> MSDQPRPTVIITGASSGVGLYATKALANRGWHVIMACRNLEKAEQAAKNLQIPPEAYTILHLDLSSLASVRGFVESFRALNRPLRALVCNAAVYYPLLKEPIYSVDGYEITVATNHLGHFLLINLLL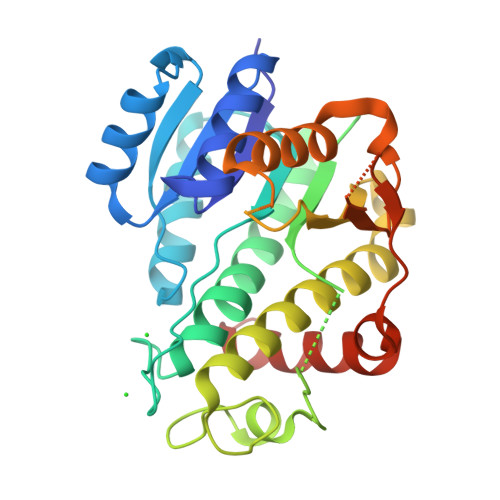EDLKNSPESDKRLVILGTVTANRKELGGKIPIPAPPDLGNLEGFEKGFKKPIAMINGKPFKSGKAYKDSKLCNMLTARELHRRFHESTGIVFNSLYPGCVADTPLFRHHFPLFQKLFPLFQKKITGGYVSQELAGERVAMVVADPEFRQSGVHWSWGNRQKEGRKAFVQELSAEASDEQKARRLWELSEKLVGLALEHHHHHH The PBP architecture consists of two opposing lobes, with each lobe being built of a central, five‐stranded parallel β‐sheet with five α‐helices flanking its sides. Despite diversity in the sequences of different PBPs, a shared common ancestry has been proposed a while ago (Fukami‐Kobayashi et al., 1999; Louie, 1993). Their structural features, similarities in binding mechanism, and shared operon structure—with the PBP being on the same operon as the associated signaling proteins downstream—have long led to the theory that PBPs arose via gene duplication of a progenitor protein and subsequent diversification. To further substantiate the claim, we biophysically and structurally characterized truncated constructs of the ribose‐binding protein (RBP) from Thermotoga maritima that correspond to the proposed duplicated progenitor halves. The two independent halves appear to readily form a heterodimer, while also reconstituting the ribose‐binding ability of the parental protein, with affinities in the same order of magnitude.

We therefore decided to continue the investigation with the truncated construct RBP‐Trunc (residues 142–310) instead, which is related to the RBP‐C half and expressed solubly with similar stability to the N‐terminal construct RBP‐N. For this, the individually purified RBP‐N and RBP‐Trunc were mixed in an equimolar ratio and then analyzed. The x‐ray structure of the heterodimer closely resembles the parental protein. The heterodimer displays the same opening and twisting angle as the paternal protein, an important indicator of a native‐like configuration of the heterodimer. The asymmetric unit of the crystal structure shows a dimer of RBP‐N/RBP‐Trunc heterodimers, which is in agreement with the oligomeric state observed in SEC‐MALS experiments; however, further analysis is needed to determine the precise conformation of the dimer of heterodimers in solution. The observed heterodimer interface in the asymmetric unit is mostly related to the interaction of C‐terminal residues of RBP‐Trunc located in the hinge region and their corresponding ones in the crystallography mates, ruling out the possibility that dimerization results from the extra elements left out in RPB‐Trunc. Finally, a closer look at the side‐chains involved in ribose binding reveals an almost identical orientation compared to the unliganded state of the native RBP, suggesting the correct formation of the preformed binding site. The results show that the halves have native‐like properties, that interdomain interactions are important in RBP and that these provide relevant stabilization, in the same way as has been described for other multidomain proteins (Brandts et al., 1989; Careaga et al., 1995; Kantaev et al., 2018; Liu et al., 2019; Vergara et al., 2023; Vogel et al., 2004; Wenk et al., 1998).

>MKGKMAIVISTLNNPWFVVLAETAKQRAEQLGYEATIFDSQNDTAKESAHFDAIIAAGYDAIIFNPTDADGSIANVKRAKEAGIPVFCVDRGINARGLAVAQIYSDNYYGGVLMGEYFVKFLKEKKLEHHHHHH[2x];>[2x]MGEYFVKFLKEKYPDAKEIPYAELLGILSAQPTWDRSNGFHSVVDQYPEFKMVAQQSAEFDRDTAYKVTEQILQAHPEIKAIWCGNDAMALGAMKACEAAGRTDIYIFGFDGAEDVINAIKEGKQIVATIMQFPKLMARLAVEWADQYLRGERSFPEIVPVTVELVTRENIDKYTAYGRKLEHHHHHH> GMDERAQAALDALLSAKNLRDVCPETVRRVFMELLPRYRKPKDAEKAARTHLHQITGAFMTADAQK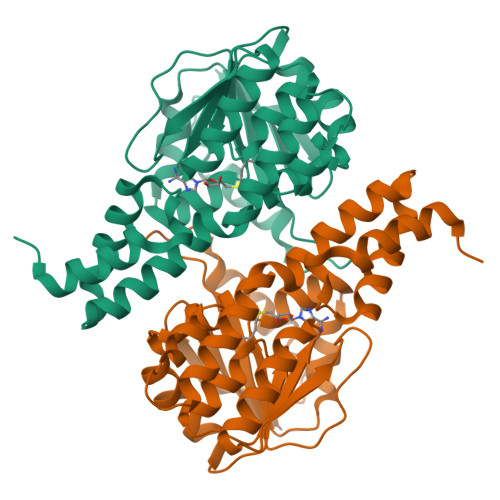KARALLARWNEGDESALAAALSLHASTRERLPGADEWMRRVSPFLGADARVLDLACGLNPILLGSMGVTNALGMDIHLGCVRLVNETARARGWHTRARACDLLSEIPAEEADAALLMKLLPVLEAQKTGRAAELLASLRAPRLVVTFPTRTLGGRGVGMEKHYADWFERILPDTLSVRDRFTVSDELVYLVERT3-(2-chlorophenyl)-5-methyl-N-[4-(propan-2-yl)phenyl]-1,2-oxazole-4-carboxamide 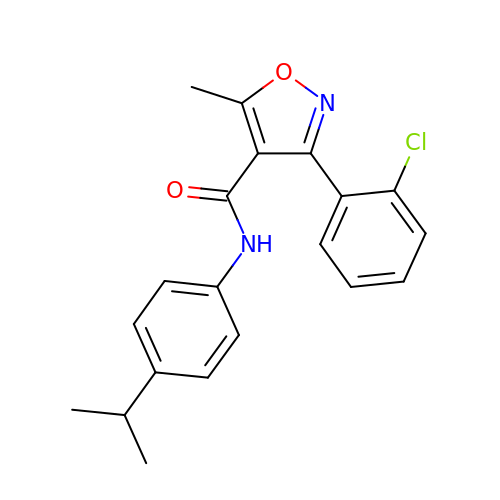| C20 H19 Cl N2 O2 | WRQYTVUHKWFTAU-UHFFFAOYSA-N>[3x]PKRGKKGAVAEDGDELRTEPEAKKSKTAAKKNDKEAAGEGPALYEDPPDQKTSPSGKPATLKICSWNVDGLRAWIKKKGLDWVKEEAPDILCLQETKCSENKLPAELQELPGLSHQYWSAPSDKEGYSGVGLLSRQCPLKVSYGIGDEEHDQEGRVIVAEFDSFVLVTA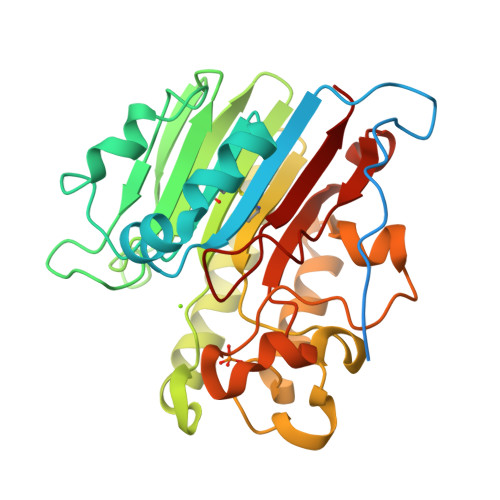YVPNAGRGLVRLEYRQRWDEAFRKFLKGLASRKPLVLCGDLNVAHEEIDLRNPKGNKKNAGFTPQERQGFGELLQAVPLADSFRHLYPNTPYAYTFWTYMMNARSKNVGWRLDYFLLSHSLLPALCDSKIRSKALGSDHCPITLYLAL>[2x]GMKL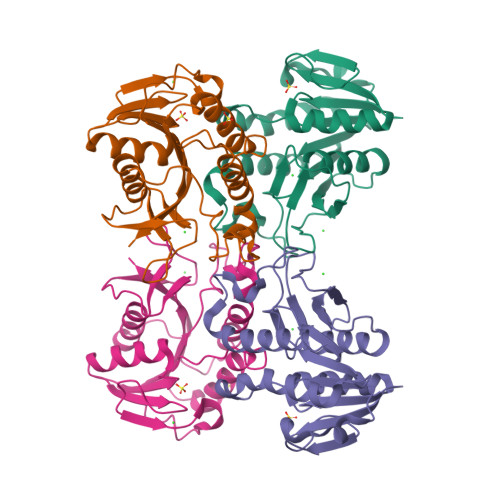AVIAANGQAGKAIVEEAVKRGHEVTAIVRSENKSQAESIIKKDLFELTKDDLTGFDAVISAFGAYTPDTLPLHSKSIELFNQLLAGTQTRFLVVGGAGSLYIDETKTTRLLDTPDFPEEFKPLAKAQADELDLLRTKNNLNWTFVSPAVDFIPDGEKTGNYILAGEIFTTNEKGISQISYADYAIGLVDELEKGHHIKERISLLEK>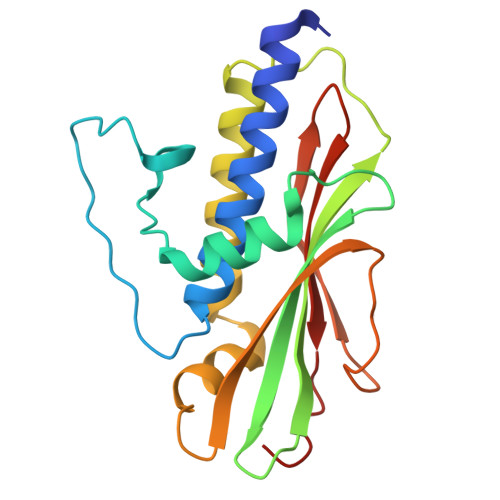 METDLNSQDRKDLDKFIKFFALKTVQVIVQARLGEKICTRSSSSPTGSDWFNLAIKDIPEVTHEAKKALAGQLPAVGRSMCVEISLKTSEGDSMELEIWCLEMNEKCDKEIKVSYTVYNRLSLLLKSLLAITRVTPAYRLSRKQGHEYVILYRIYFGEVQLSGLGEGFQTVRVGTVGTPVGTITLSCAYRINLAFMS1-ethyl-1H-benzimidazole | C9 H10 N2 | 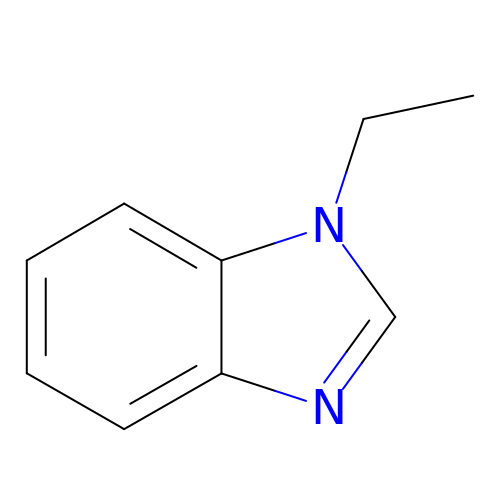WVNMLOGVAVGQIT-UHFFFAOYSA-N> MLHVVQLDDFATRLKAAEDYQSKHSVLSEICDSLETFNAAQDYEYFLKSLIPLFIDVLKEVPVSFVANSPENKLRNITLEILHRIPANDALQAYSNEIVDTLMDLLKVENELNGILCMKAITTLHKTFKASLQEKVHPFIDIVIEIYSNIPQVVEEQFNGNQIDSKENVDSTSRPNSPSFSSQSDDSKQLAQAMFSFKTLAESPITMVSLYSSYKELAASSLGNFIPHVMKVLSLEVAKQAEARKAAEEKGIILVNVCKEITNRANYGEFIIGQVKAASFLAYLFIRRQAQTFLEPYQQAIPDIIIRLLQDCPSELSAARKELLHATRHILSTDFRKMFIPKIDLLFDLRVLIGEGFTAYETLRPLAYSTVADFIHNVRDHLTPAQLWKSVSIYCKNLQDDSLALTVQIMSAKLLLNLIEKIMRSESKTESRQLLMVIIDAYTKRFKMLNSRYNGIMKQHATYEKEKQEKQNQERLLTNKLDGTTPSPSDDKKVELIDEDQDVKMEDPTPEISDQETIKGDNDASTEPQDSEQQLADFMSLQEYLPIQVSVPPEIDLLKDSRYLFKTLMTFLKTIMIGLKNSNPPSSQNHFNAQNWNETARGFSNEDINILKSLFRECILALRFFSTSKTSLPASSMKQSFDITGPNLPITSTKEEKDLMEIFATMFIHIDPASFNEIVREELPFMYKQMLDFASLLHIPQFFLASVITSSSFSGILITFLKSKLVDLGEVNIIKSNILIRLFKLCFMSVSLFPAANESVILPHLNELILKSLKLSTTAKEPLVYFYLIRTLFRSIGGGRFENLYKEIMPLLQVLLESLSKLIHEARRPQERDIYVELCLTVPVRLSVLVPHLSYLMKPLVYALNGSQESVSQGLRTLELCVDNLTAEYFDPIIEPVIDDVMEALSKHLKPLPYYHQHSHTTLRILGKLGGRNRTFIKPVDNLKTDSELFQNVEAMFKIHGLPNEVPLSITPGLSAAFSLLTDPRPRIHYRINSFKYISGIFQLFLGATQLPDDYANRLKESMDIILEDTIAPDEPLNKLHHFPVKDIAKYDSQMELLVKLLESIFYAVSLQEVREESKALIRGTCNHFILLYFNKMVIDKRKFVRKFSVDNHEGNLFLNENCIFDAIIYALSSDNSAVRSMGLESVQLIYDSCVELFGNIDCALKFAPLNVMCSKFIHCCFEEPYHKKLAGCIGLEMMLNSLDIPMKYFNARQLEIIRALFYVLRDTAPELPCEVTNTAKRLILNSLKEWNKELTRNDVFSSVFQNLVSSLIVDLPNANEIVRATAQEALRTLSETTQVPIATMISPCKHILLAPIFGKPLRALPFQMQIGNIDAITFCMGLENSFLEYNEELNRLVQEALALVDAEDESLVSAHRISEHKTSEQLVRLRVVCIQLLSLAITKPEFAAAQQRSNIRVKILVVFFKSLCGRSIEIIRAAHGGLKAVIDLKMKLPKELLQNGLRPMLMNLSDHKKLTVASLEALSGLLKLFISYFKVGIGSKLLDHLLAWAQPRTLQQLGSQDLENNSTVQIIVAILDVFHLLPPTAHKFMNDLMNALLYLENNLHRCQYSPFREPLAKFLDRFPDESFEYFFNEFSKREITTRFVYFVGLDSCSSLRAKVLESLPRVRGLLHQEGSAEEKCVRFSNLVDLCESLAASDKEWIKDKEELLGELLDAGSVCLTLKRSSNVVSPLYFQVDQGFETLQLLYIEYFKSQPLGHEKVFNFIDKISKEGLPFVLEFDDFIFNEVVKCQDIPTVQQTLDTIIRMTPQVSSLDARVYLYKRIFLPICIYESEMHGDLSRLSQTENNELPAWLKSFDSDVWKATGPLVDDYTSTLEDRYRLELMQLTALLIKGAPTALTDMRKDIIKFSWNYIKLDDNTSKQAAYVVTAYFISRFDTPSELTTRIFVALLRCHQIDTRYLVKQALELLAPVLSERTNSELDWLKWPRRVLSEDGFNITQVANIYQLIVKFPDLFYPARDHFIPNIITAMGKLTVMSNTSLENQQLAIDLAELILKWETKLPKSEKLGSAEETEKEKSVSEDKMDIDVKEETKEDIAERPKAEDQIGGDDSDSSNILTSEDYEVSFAQREACVTFLIRYICISTQRPSENELGKRALNILYELLGPKYWSEVTVKLQFFERFLMSSDLNQPSLLGYCLNALEVLAVALKWKPTTWIIENVSYLQKLLEKCLRSDNQDIQEILQKVLGIILEAINKETQGSEEDEPEEVTNFISLIVNIIGEDLSNMTSVAAGVSLCWTLSLYRPNALDSLLPSIMRTFNKLCRDHIAISLQGNQPQSGDFANIEFEAKVTTNLLEKILNLCAARISSLDDQRRVFLSLLAQLIDRSVDKDMLLKVINIVTEWIFKTDFYPTTKEKAGILGKMMIFDLRGEPELSKKFNQVIVDIFESKELAHTELTARMETAFLFGTRLSDVSIRKKLMSILSDSLELDIDKRLFYIIKDQNWEYLSDYPWLNQALQLLYGSFHLDSPIRLSPEENTLSPLQSITEGLAREKSPVEKAPQNIIDFVAKHNEFLDSVRSLTAGDILNPLIDISYQSAETIHNAWVVVFPVAYSAIESRYELEFTRALVKLLFKDYHIRQQDARPNVIKSLLDGVGKCPGLHLPPHLVKYLGSNYNAWYGAIKLLEELSEGQGIDNQKISDANQDALLEVYMSLQEDDMFYGTWRRRAKYFETNAALSYEQIGIWDKALQLYEAAQIKARSGVFPFGESEYSLWEDHWIYCAEKLQHWEILTELAKHEGFTDLLLECGWRGADWIADREPLEQSVKTVMDIPTPRRQIFQTFLALQGFSQQKDTLQDVSRLCDEGIQLTLRKWNALPQRVTRAHIGLLHTFQQYVELMEASQVYSSLVTTNAQNLDVKSQELKRVLQAWRERLPNVWDDINIWNDLVTWRQHVFGVINRVYMPFVPVLQQSNGTNNGNSYAYRGYHEMAWVINRFAHVARKHEMPEVCINQLTKIYTLPNIEIQEAFLKLREQAKCHYQNSSELNTGLDVISNTNLVYFATQQKAEFFTLKGMFLAKLNAKDEANQAFATAVQIDLNLPKAWAEWGFFNDRRFKENPEEIFHAKNAISCYLQAAGLYKDGKTRKLLCRILWLISLDDAAGSLAKTFEDHHGESPVWYWITFVPQLLTSLSHKEAKIVRHILIQIAKSYPQSLHFQLRTTKEDYQAIQRQAMAVNRAEEQSSNK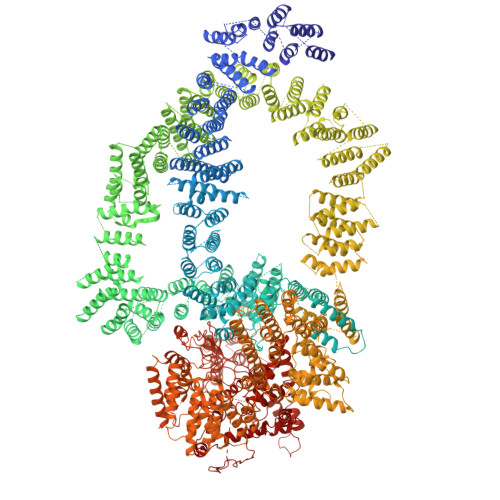QDTADSVLKNTNTPQPQTRTETSGTTAESDKKPSIPPKEEQGSPQPSRPATTQASPQAQSQENGESSQKHPPEIPTTDSRQPWQDVEEIMGILKTAYPLLALSLESLVDQLNQRFKCNADEDAYRLVIVLYNDGVQQMNRVANPREEVKLPAATEASISRFADSVLPKNIREVFEQDIIACNPNLETYISKLRKWRDCLEEKLDRSYGKADLERVSLHLSLFHHQKFEDIEIPGQYLLHKDNNNHFIKIERFLPTLDLVRGSNGCYKRMTIRGNDGSLHPFAVQFPAARHCRREERIFQLFRIFDDALSRKVQSRRRNISLTLPIAVPLSPHIRILNDDKRYTTLMGIYEEFCRRKGQSRDEPFAYTIQKLRAAFDPRLPKPDIVSVRAEVLASIQSTLVPSTLLKDYYTEKFSNYENYWLFRKQFTAQYASFIFMTYIMCINSRQPQKIHINEGSGNIWTSEMLPTKVATGKTHSTAYNNSTLDPAVKAGAPIFYNTESVPFRLTPNIQKFIGEAGLEGILSVYILVIANSLSDSEFDMEQYLSLFVRDEVISWFAQQHRASAQTNQLREIVRVNVELLTKRVLQLNHIPNSQNVATQFVLNLISQAVNPRNLAYTDSAWMAYL>MSLSKKRKLESGDSGGAGAGGEGAEEENGGEQEAAPPRPRRTKSERDQLYYECYSDVSVHEEMIADQVRTEAYRLGILKNWAALRGKTVLDVGAGTGILSIFCAQAGARRVYAVEASAIWQQAREVVRLNGLEDRVHVLPGPVETVELPERVDAIVSEWMGYGLLHESMLSSVLHARTKWLKEGGLLLPASAELFVAPISDQMLEWRLGFWSQVKQHYGVDMSCMESFATRCLMGHSEIVVQDLSGED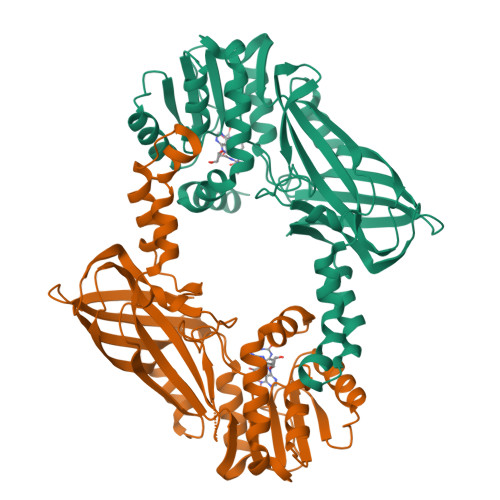VLARPQRFAQLELARAGLEQELEAGVGGRFRCSCYGSAPLHGFAVWFQVTFPGGDSEKPLVLSTSPLHPATHWKQALLYLNEPVPVEQDTDISGEITLLPSPDNPRRLRILLRYKVGDHEEKTKDFAMEDGSENLYFQG[2x]The enzyme CdaA, which synthesizes an essential second messenger cyclic di-AMP (c-di-AMP) in many pathogenic bacteria, has emerged as a promising candidate for the development of novel antibiotics. Additionally, c-di-AMP regulates the bacterial stringent response, further underscoring its significance. The synthesis of c-di-AMP is mediated by enzymes possessing a diadenylate-cyclase (DAC) domain.

To identify crystals suitable for fragment screening, CdaA enzymes from Streptococcus pneumoniae, Bacillus subtilis and Enterococcus faecium were purified and crystallized. Crystals of B. subtilis CdaA, which diffracted to the highest resolution of 1.1 Å, were used to perform the screening of 96 fragments, yielding data sets with resolutions spanning from 1.08 to 1.87 Å. Additionally, we report the first crystal structures of apo CdaA from E. faecium (EfCdaA) and S. pneumoniae (SpCdaA), as well as atomic resolution structures of BsCdaA. Evaluation of the tested CdaA crystals from three different bacteria revealed that the BsCdaA crystals were the most suitable for fragment screening. Consequently, we selected B. subtilis CdaA for the fragment-screening campaign due to the excellent diffraction properties, high reproducibility and quality of BsCdaA crystals. Notably, these crystals tolerated up to 20% DMSO in the reservoir solution, which facilitates soaking experiments. In conclusion, we have demonstrated that a structurally related enzyme from a nonpathogenic bacterium can be used to identify crystallization conditions that yield crystals suitable for a crystallographic fragment-screening campaign.

>GPTPVEEAQQKTIEAITKAINYMAKRRIGALLTIERDTGMGDYIETGIPLNAKVSSELLINIFIPNTPLHDGAVIMKNNEIAAAACYLPLSESPFISKELGTRHRAAVGISEVTDSLTIIVSEETGGVSVAKNGDLHRELTEEALKEMLEAEFK[2x]>MQQKYQPTEANLKARSEFQDNKFGIFLHWGLYAMLATGEWTMTNNNLNYKEYAKLAGGFYPSKFDADKWVAAIKASGAKYICFTTRHHEGFSMFDTKYSDYNIVKATPFKRDVVKELADACAKHGIKLHFYYSHIDWYREDAPQGRTGRRTGRPNPKGDWKSYYQFMNNQLTELLTNYGPIGAIWFDGWWDQDINPDFDWELPEQYALIHRLQPACLVGNNHHQTPFAGEDIQIFERDLPGENTAGLSGQSVSHLPLETCETMNGM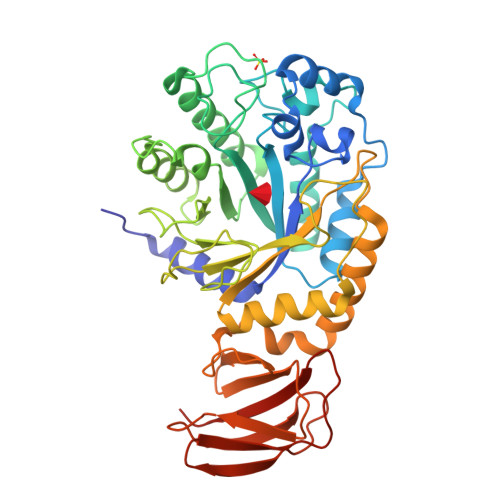WGYKITDQNYKSTKTLIHYLVKAAGKDANLLMNIGPQPDGELPEVAVQRLKEVGEWMSKYGETIYGTRGGLVAPHDWGVTTQKGNKLYVHILNLQDKALFLPIVDKKVKKAVVFADKTPVRFTKNKEGIVLELAKVPTDVDYVVELTIDDEHHHHHH[2x]>[2x]MRGKIYDRNGKVLAEDVERYKLVAVIDKKASA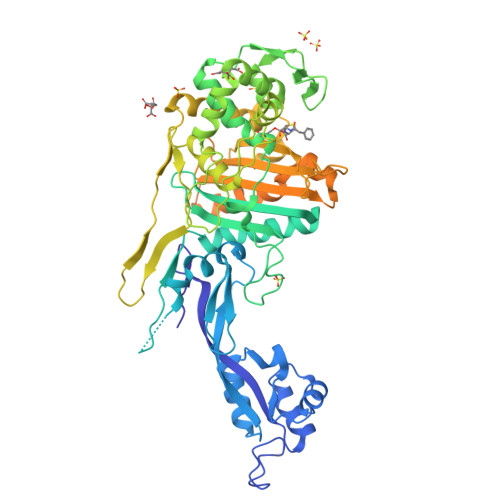NSKKPRHVVDKKETAKKLSTVINMKPEEIEKRLSQKKAFQIEFGRKGTNLTYQDKLKIEKMNLPGISLLPETERFYPNGNFASHLIGRAQKNPDTGELKGALGVEKIFDSYLSGSKGSLRYIHDIWGYIAPNTKKEKQPKRGDDVHLTIDSNIQVFVEEALDGMVERYQPKDLFAVVMDAKTGEILAYSQRPTFNPETGKDFGKKWANDLYQNTYEPGSTFKSYGLAAAIQEGAFDPDKKYKSGHRDIMGSRISDWNRVGWGEIPMSLGFTYSSNTLMMHLQDLVGADKMKSWYERFGFGKSTKGMFDGEAPGQIGWSNELQQKTSSFGQSTTVTPVQMLQAQSAFFNDGNMLKPWFVNSVENPVSKRQFYKGQKQIAGKPITKDTAEKVEKQLDLVVNSKKSHAANYRIDGYEVEGKTGTAQVAAPNGGGYVKGPNPYFVSFMGDAPKKNPKVIVYAGMSLAQKNDQEAYELGVSKAFKPIMENTLKYLNVGKSKDDTSNAEYSKVPDVEGQDKQKAIDNVSAKSLEPVTIGSGTQIKAQSIKAGNKVLPHSKVLLLTDGDLTMPDMSGWTKEDVIAFENLTNIKVNLKGSGFVSHQSISKGQKLTEKDKIDVEFSS> MARAMAAAWPLLLVALLVLSWPPPGTGDVVVQAPTQVPGFLGDSVTLPCYLQVPNMEVTHVSQLTWARHGESGSMAVFHQTQGPSYSESKRLEFVAARLGAELRNASLRMFGLRVEDEGNYTCLFVTFPQGSRSVDIWLRVLAKPQNTAEVQKVQLTGEPVPMARCVSTGGRPPAQITWHSDLGGMPNTSQVPGFLSGTVTVTSLWILVPSSQVDGKNVTCKVEHESFEKPQLLTVNLTVYY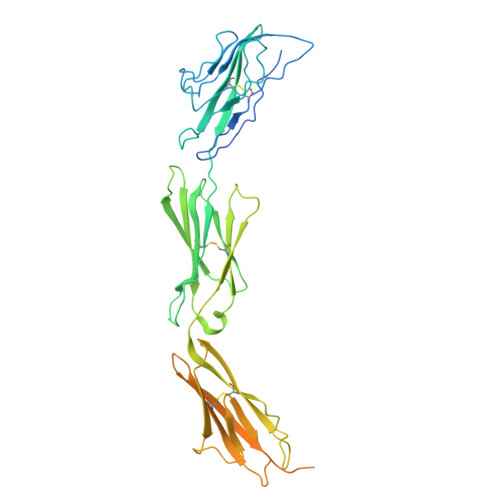PPEVSISGYDNNWYLGQNEATLTCDARSNPEPTGYNWSTTMGPLPPFAVAQGAQLLIRPVDKPINTTLICNVTNALGARQAELTVQVKEGPPSEHSGISRNAIIFLVLGILVFLILLGIGIYFYWSKCSREVLWHCHLCPSSTEHASASANGHVSYSAVSRENSSSQDPQTEGTRHHHHHH>MSRNTEATDDVKTWTGGPLNYKEGFFTQLATDELAKGINEEVVRAISAKRNEPEWMLEFRLNAYRAWLEMEEPHWLKAHYDKLNYQDYSYYSAPSCGNCDDTCASEPGAVQQTGANAFLSKEVEAAFEQLGVPVREGKEVAVDAIFDSVSVATTYREKLAEQGIIFCSFGEAIHDHPELVRKYLGTVVPGNDNFFAALNAAVASDGTFIYVPKGVRCPMELSTYFRINAEKTGQFERTILVADEDSYVSYIEGCSAPVRDSYQLHAAVVEVIIHKNAEVKYSTVQNWFPGDNNTGGILNFVTKRALCEGENSKMSWTQSETGSAITWKYPSCILRGDNSIGEFYSVALTSGHQQADTGTKMIHIGKNTKSTIISKGISAGHSQNSYRGLVKIMPTATNARNFTQCDSMLIGANCGAHTFPYVECRNNSAQLEHEATTSRIGEDQLFYCLQRGISEEDAISMIVNGFCKDVFSELPLEFAVEAQKLLAISLEHSVG[2x];>[2x]MAGLPNSSNALQQWHHLFEAEGTKRSPQAQQHLQQLLRTGLPTRKHENWKYTPLEGLINSQFVSIAGEISPQQRDALALTLDSVRLVFVDGRYVPALSDATEGSGYEVSINDDRQGLPDAIQAEVFLHLTESLAQSVTHIAVKRGQRPAKPLLLMHITQGVAGEEVNTAHYRHHLDLAEGAEATVIEHFVSLNDARHFTGARFTINVAANAHLQHIKLAFENPLSHHFAHNDLLLAEDATAFSHSFLLGGAVLRHNTSTQLNGENSTLRINSLAMPVKNEVCDTRTWLEHNKGFCNSRQLHKTIVSDKGRAVFNGLINVAQHAIKTDGQMTNNNLLMGKLAEVDTKPQLEIYADDVKCSHGATVGRIDDEQIFYLRSRGINQQDAQQMIIYAFAAELTEALRDEGLKQQVLARIGQRLPGGAR;>[4x]MLSIKDLHVSVEDKAILRGLSLDVHPGEVHAIMGPNGSGKSTLSATLAGREDYEVTGGTVEFKGKDLLALSPEDRAGEGIFMAFQYPVEIPGVSNQFFLQTALNAVRSYRGQETLDRFDFQDLMEEKIALLKMPEDLLTRSVNVGFSGGEKKRNDILQMAVLEPELCILDESDSGLDIDALKVVADGVNSLRDGKRSFIIVTHYQR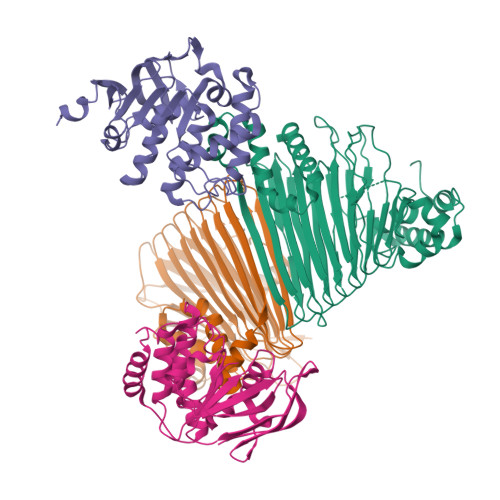ILDYIKPDYVHVLYQGRIVKSGDFTLVKQLEEQGYGWLTEQQ>QTVTGGLRSLYQRKVLPLEEAYRFHEFHSPALEDADFENKPMILLVGQYSTGKTTFIRYLLEQDFPGMRIGPEPTTDSFIAVMYGETEGSTPGNALVVDPKKPFRKLSRFGNAFLNRFMCSQLPNQVLKSISIIDSPGILSGEKQRISRGYDFCQVLQWFAERVDRIILLFDAHKLDISDEFSEAIKAFRGQDDKIRVVLNKADQVDTQQLMRVYGALMWSLGKVINTPEVLRVYIGSFWAQPLQNTDNRRLFEAEAQDLFRDIQSLPQKAAVRKLNDLIKRARLAKVHAYIISYLKKEMPNMFGKENKKRELIYRLPEIYVQLQREYQISAGDFPEVKAMQEQLENYDFTKFHSLKPKLIEAVDNMLTNKISSLMGLISQEEMNMPTQMVQGGAFDGTTEGPFNQGYGEGAKEGADEEEWVVAKDKPVYDELFYTLSPINGKISGVNAKKEMVTSKLPNSVLGKIWKLADCDCDGMLDEEEFALAKHLIKIKLDGYELPNSLPPHLVPPSHRK[16x]

Eps15-homology domain containing proteins (EHDs) are eukaryotic, dynamin-related ATPases involved in cellular membrane trafficking. EHDs harbor a dynamin-related GTPase (G-) domain that binds to adenine rather than guanine nucleotides. EHDs tubulate negatively-charged liposomes in an ATP-dependent manner by the formation of ring-shaped and helical filaments on the remodeled membranes. EHD4/Pincher mediates macropinocytosis required for retrograde endosomal Trk signaling.

In the present work, we reconstitute an N-terminally truncated EHD4 variant on tubular membrane templates and determine these structures by cryo-electron tomography (cryo-ET) and subtomogram averaging (STA). Accordingly, our in vitro reconstitutions were done in the presence of the nonhydrolysable ATP analogue, adenylyl-imidodiphosphate (AMPPNP). The resulting cryo-electron microscopy (cryo-EM) density map had an average resolution of 7.6 Å and 8.5 Å, as determined by FSC and FSC-independent analyses, respectively. EHD4 formed right-handed helical filaments wrapping around the lipid tubes. The EH domains are located furthest from the membrane, the G-domains at the center and the helical domains closest to the membrane. As in the previously reported crystal structures, dimerization of EHD4 is mediated by helix α6 in the G-domain. Interface-2 is formed between the helical domain of one protomer and the G-domain of the adjacent protomer along the filament. Interface-3 is formed between G-domains of two adjacent dimers across the filament and corresponds to the archetypal G-interface that is conserved in all members of the dynamin family. Membrane-bound EHD4 adopted the closed conformation of the helical domain, akin to the reported EHD2 conformation. Thus, helices α8 and α9 in the helical domain engage with the membrane bilayer by inserting hydrophobic residues at the connecting loop into the membrane outer leaflet.Imidazoleglycerol-phosphate dehydratase (IGPD) catalyzes the Mn(II)-dependent dehydration of imidazoleglycerol phosphate (IGP) to 3-(1H-imidazol-4-yl)-2-oxopropyl dihydrogen phosphate during biosynthesis of histidine. The metalloenzyme imidazoleglycerol-phosphate dehydratase (IGPD) (EC 4.2.1.19) has been identified as a potential herbicide target due to its essential role in histidine biosynthesis (Ames, 1957; Hilton et al., 1965). Since the substrate lacks a carbonyl or imine adjacent to the leaving proton, which is thus non-acidic, IGPD uses an unusual mechanism for catalysis that is distinct from other dehydration reactions that have been reported to date (Glynn et al., 2005).

To provide a foundation on which to analyze substrate binding, we determined the structure of A. thaliana IGPD isoform 2 (IGPD2) in complex with inorganic phosphate (1.75 Å resolution), which is a weak inhibitor of the enzyme (Ki ∼5 mM) (Wiater et al., 1971a). The native protein crystallized as the same 24mer species that has been observed previously, and this structure shows that within the active site of the holoenzyme, both of the Mn(II) ions are octahedrally coordinated by four conserved protein ligands and two water molecules; HOH3/HOH4 for Mn1 and HOH1/HOH2, for Mn2. The holoenzyme has an open conformation where the C-terminal region (R193–R206, termed the C loop), which contains a number of conserved residues, is disordered.

>SPIESARIGEVKRETKETNVSVKINLDGHGVSDSSTGIPFLDHMLDQLASHGLFDVHVRATGDTHIDDHHTNEDVALAIGTALLKALGERKGINRFGDFTAPLDEALIHVSLDLSGRPYLGYNLEIPTQRVGTYDTQLVEHFFQSLVNTSGMTLHIRQLAGKNSHHIIEATFKAFARALRQATESDPRRGGTIPSSKGVLSRS[8x]Here, we obtained the true atomic resolution structure of their methane-capturing system (Methyl-Coenzyme M Reductase, MCR), circumventing the isolation barrier by exploiting microbial enrichments of freshwater nitrate-reducing ANME-2d grown in bioreactors, and marine ANME-2c in syntrophy with bacterial partners. Methane capture, the first reaction in AOM, has been proposed to be carried out by the Methyl-Coenzyme M Reductase (MCR). In the proposed mechanism, the heterodisulfide, made of Coenzyme M (HS-CoM) and Coenzyme B (CoB-SH), would react with methane to generate methyl-S-CoM and free CoB-SH through a radical mechanism catalysed by the Ni-containing tetrapyrrole cofactor F43019,20. Despite their physiological differences, these ANMEs have extremely conserved MCR structures, similar to homologs from methanogenic Methanosarcinales, rather than the phylogenetically distant MCR of ANME-1 isolated from Black Sea mats.

X-ray crystal structures were solved for MCR from ANME-2dO and ANME-2dV, and models were refined to a final resolution of 0.98 Å. The subatomic resolution of both ANME-2d structures enables the visualisation of the majority of hydrogen atoms and accurately depicts the position of each ligand atom. However, MCR from ANME-2dV exhibits a mixture of ligands. The fit to the electron density was optimal when the model included CoM-SH, CoB-SH, the heterodisulfide, and methyl-CoM. The methyl-CoM, modelled for the first time in an experimental structure, fits a position proposed in a recent molecular dynamics simulation model by Polêto and colleagues with a S–Ni distance of 3.9 Å36. However, due to its low occupancy and the requirement for experimental validation to confirm its existence, we omitted the methyl-CoM from the final deposited model. In both ANME-2d, a canonical glutamine (position α341 in ANME-2c), proposed to be important to anchor the F430, and juxtaposed to the tyrosine coordinating the CoM thiol (position α342 in ANME-2c), is substituted by a methionine (positions α343 and α347 in ANME-2dO and ANME-2dV, respectively). The substitution does not impact the F430 position and provokes few steric displacements in the vicinity. The three studied enzymes have seven post-translational modifications, among them was a novel 3(S)-methylhistidine on the γ-chain of both ANME-2d MCRs. The location of the 3(S)-methylhistidine interacting directly with F430 suggests a compensation for the lack of the methylglutamine in ANME-2dO and ANME-2dV placed in a close proximity.

>[2x]MAEPRFKKSMETKYAKEWGSNKVGSTAKAKITDKKTKYLRLGYQQNPRKVEMAKCGAAITKKRGLQAYDPKLHLAGIPMGQRQLTPYTISGTDIVCDGDDLHFVNNAAMQQEWDDIRRTCVVGLDLAHETLEKRLGKEVTPETINYYLEVLNHAMPGAAIVQEHMVETHPALVDDCYVKIFTGDETLQDEVDKQFVINIDNEFPANQAKQIKAAVGKTSWQAVHIPTIVTRTEDGPGTSRWMAMQVGMTFISAYHMCAGEAAVGELAFTAKHAGLVEMGDMIPARRARGPNEPGGLSFGHMADIVQTNRKGPEDPVNVVLQTASAATMLYDQIWLGGYMSGGVGFTMYATPAYTNDIVDDFLYWGNDYAAKKYGGNGKAKATIDTVKDIATETTLYGLEAYEKYPTTLEDHFGGSQRATVISIAAGGATALATGHSQAGLSAWYLSMYLHKEAHGRLGFYGYDLQDQCGATNVFSIASDEGCIGECRGANYPNYAMNVGHQGGYTSVVAAAHAGKDAFCVNPLVKTCFADELINFDFADPRAAFGKAALREWDRCAGERAFVIPAK;>MADTIDLYSDRGAKLKSGVDINDISPMRNAAIKSIVTGIKRTAAVDLAGIEKTLATSAIGGKGRKIPGREMKLDIVKNAAAIQKAVNELVQVDSGDDTVVKALNGGKQLIVQVPSVRIDVAAEYVSSLTCTASAVTQALVSQFNIGMFDAPTIKSAVWGQYPQTLDMVGGNVKSIVDIPQKDEGFGYTLRNVMANHLAATCKKSAMNTAALCSILENTGVFEMGDAIGNQTRHRLLAFSHQGLNANNLVYGTTKALGKTGTIGSAVHACVEKAIADKVISADKKFASGYTTYKTNDVGKWNAYCAAGTLVATLINCGAQRAPQSVSAVLLYFNDLIEKETSLPGCDFGKVQGAAVGFSFFSHSIYGGGGPGVFNGNHVVTRHSKGLAVPCVAAAVALDAGVQIYSPEKTSGLVGDVFSSVDEFREPIKAVAGAV[2x];>MAYKPQYYPGSTSVAKNRRKHMSDDVEKMRDISDEDLTALLGHRAPGSDYPSTHPPLSEIGEPACSVREVVEPTPGAAAGDRLRYVQWSDSMYNAPSVPYWRSYHAAINFRGVDPGTLSGRQVNEMRERDMEEYAKRQAETEMTDWGLAGMRGCTVHGXSLRLQEDGVMFDMLDRRRLEGGVIVSDKDQVGVPIDRKVNLGKPMSEAEAAKRTTFYRVDNVAFRSDKEVIEHVQKVWELRTKYGFVPKA[2x]>ADAQKAADNKKPVNSWTCEDFLAVDESFQPTAVGFAEALNNKDKPEDAVLDVQGIATVTPAIVQACTQDKQANFKDKVKGEWDKIK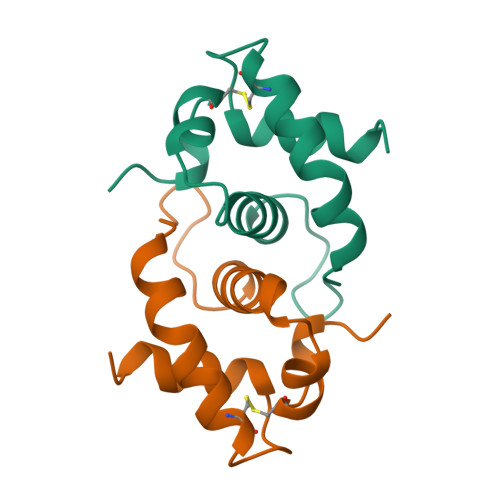KDM[3x]>AANLYYKCDVGDSVNLEEVLNMDCDAALTENRDEHPRIPTGESHKSYFFTKRACRDRLGLACYLLQVYGYPKKYQFSQYSNMEWKVC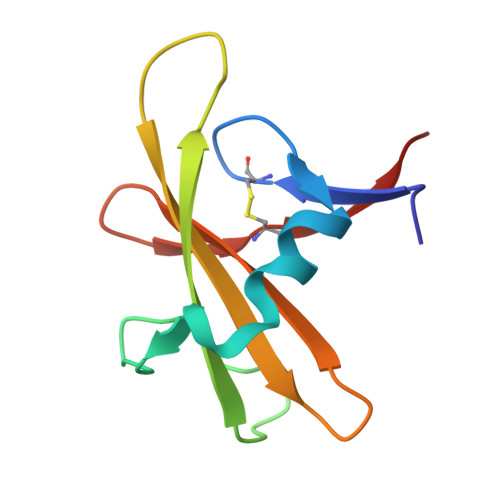SLQDIR[2x]2-acetamido-2-deoxy-6-O-sulfo-beta-D-glucopyranose | C8 H15 N O9 S | 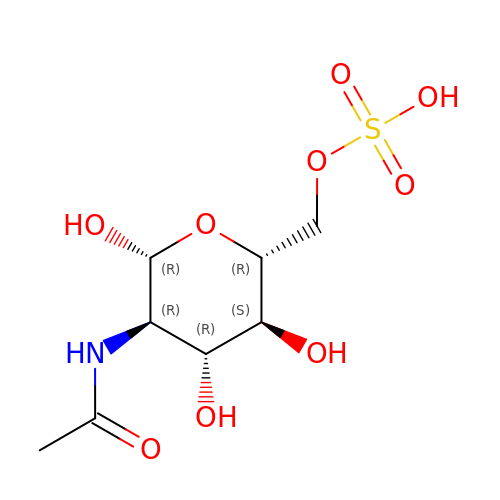WJFVEEAIYIOATH-FMDGEEDCSA-N>[3x]MCRKNRFFALAGFFLFGVFTISSC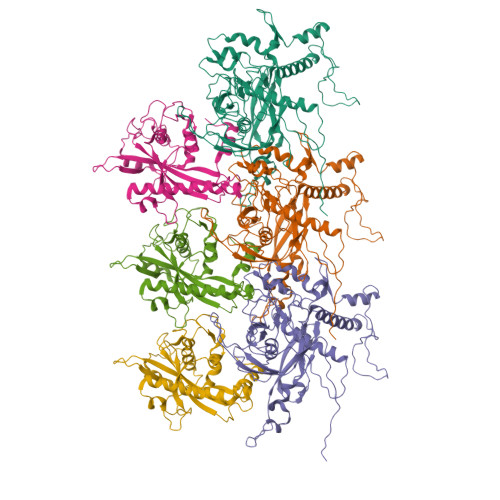GSSKRAVGGELTGAKLSSWNEPSPFGMIQVPRGSIVLGNKEADSLWGIPAESRPISVDAFWMDRTEITNAQYRQFVYYVRDSIIRERLADPAYGGNEEYKITENKFGEPVTPHLDWSKPIPSEKRATEEEIAAINSVYYTNPVTHDRKLNPDQMVYRYEVYDYRSAALREHQLKAAKRNLNTDIKVDPNAVVMISKDTAFVDESGNIISETITRPLSSEYDFLNTYIVPIYPDETCWVNDFPNARTEIYTRMYFNHPGYDDYPVVGISWEQAQAFCAWRSEFFRKGIRLPEGQIMDDFRLPTEAEWEYAARMGDSNNKYPWSTEDLRTGRGCFLGNFKPGEGDYTADGHLIPSRVSSFSPNDFGLYDMAGNVAEWTSTAFSESGLKQMSDINPELEYKAALTDPYILKQKVVRGGSWKDVARFIRSATRSHEYQNVGRSYIGFRCVRTSIAFSSGKAPKSSRRSIKK;>[3x]MKVFKAVIGAILAATVSIPSVAQENTNNRSPQVGRAPRNTEVEQMTTLSNRAQEFNRRLTQKTDNAPWRRVVYRRVDLMEESNAVLYYPPRPIGDRKNLFSTIFGLINSNSLDVYEYLDGFEAFTDQYKIKFQEFLDRFGIYYQPSTNKNAELFKVADSDIPSAEVKAYYVKEEWYFTPTNSDVDIKIQAICPIMTGQDEFGEVRNQPLFWIPYENIRPYIARERVMLSSLNNTRNSTIDDFFRLNLYKGDIVKTENLHNRALAEYCPTPDSMKMESKRIDKELQGFRDGLFVTQDTTWMKQVETKKSKGKKLEKARGKNITSRTRGQGEGAAETEAVEPKKQKASKNKAATRSVRRRK> TDNTKPNRMPVAPYWTSPEKMEKKLHAVPAAKTVKFKCPSSGTPNPTLRWLKNGKEFKPDHRIGGYKVRYATWSIIMDSVVPSDKGNYTCIVENEYGSINHTYQLDVVERS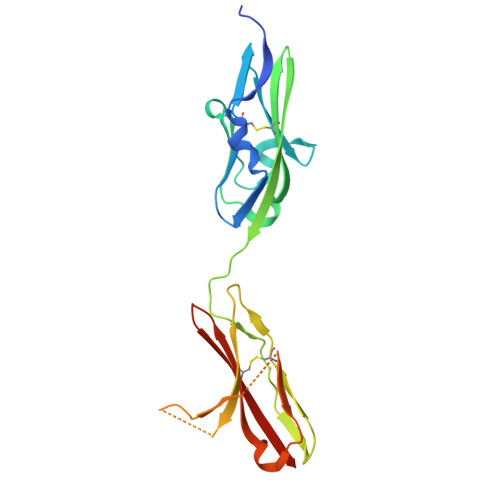PHRPILQAGLPANKTVALGSNVEFMCKVYSDPQPHIQWLKHIEVNGSKIGPDNLPYVQILKTAGVNTTDKEMEVLHLRNVSFEDAGEYTCLAGNSIGLSHHSAWLTVLEALEER>[4x]HHHKYTVITGASSGIGYETAKLLAGKGKSLVLVARRTSELEKLRDEVKQISPDS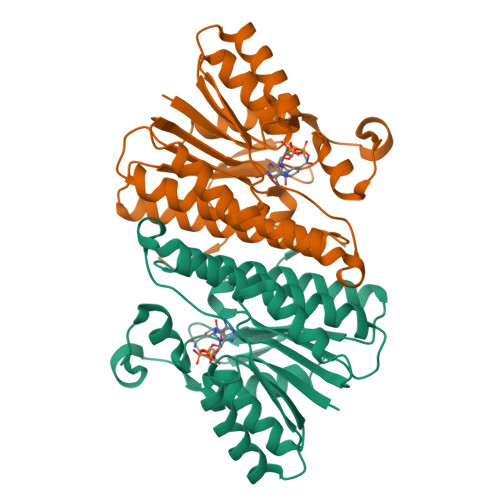DVILKSVDLADNQNVHDLYEGLKELDIETLINNAGVGDFDLVQDIELGKIEKMLRLNIEALTILSSLFARDHHDIEGTTLVNISSLGGYMIVPNAVTYCATKFYVSAYTEGLAQELQKGGAKLRAKVLAPAATETEFVDRARGEAGFDFSKAVKKYHTAAEMAGFLHQLIESDAIVGIVDGETYEFELRGPLFNYAG> HHHHHMIRPEYLRVLRKIYDRLKNEKVNWVVTGSLSF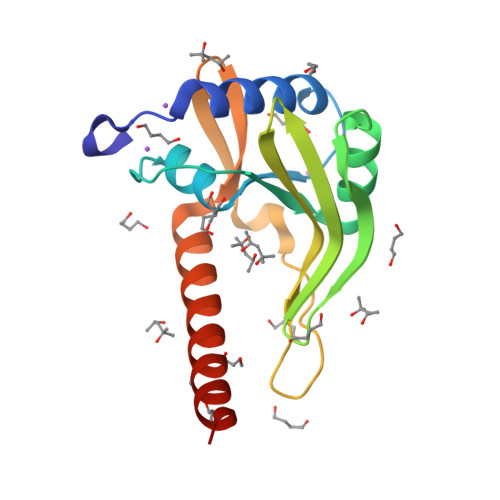ALQGVPVEVHDIDIQTDEEGAYEIERIFSEFVSKKVRFSSTEKICSHFGELIIDGIKVEIMGDIRKRLEDGTWEDPVDLNKYKRFVETHGMKIPVLSLEYEYQAYLKLGRVEKAETLRKWLNERKG lignostilbene | C16 H16 O4 | 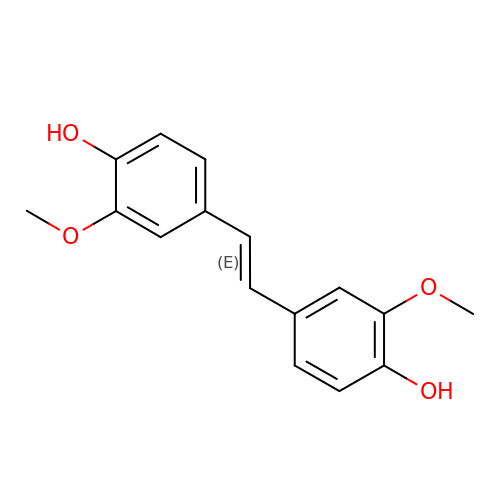KQPXJFAYGYIGRU-ONEGZZNKSA-N>GFFSFIGEAFQGAGDMWRAYTDMKEAGWKDGDKYFHARGNYDAAQRGPGGVWAAEKISDARESFQEFFGRGHEDTMADQEANRHGRSGKDPNYYRPPGLPAKY[24x]

SAA1.1 is an acute phase protein that becomes strongly upregulated during inflammation. Chronic inflammatory conditions, such as tuberculosis, leprosy and rheumatoid arthritis, are risk factors for the development of systemic AA amyloidosis. We report three cryo-EM structures of SAA1.1-derived amyloid fibrils: one that was extracted from the diseased murine tissue and two that were formed from murine SAA1.1 protein in vitro. In vitro and ex vivo fibrils possess parallel cross-β sheets but differ in their overall topologies and fibril protein folds.

Cryo-EM reconstructions achieved spatial resolutions of 2.73 Å for morphology i and 2.95 Å for morphology ii. Morphology ii is also polar but presents C2 symmetry. It consists of two PFs that both exhibit the structure of the morphology i PF. Both fibril morphologies contain an identical protein fold. In contrast to morphology i, however, morphology ii PFs contains two non-equal protein stacks, termed here stacks a and b. They differ in their relative position in the fibril structure and at the interface between the two PFs. Lys24 (stack a) in one PF is packed against Glu25 (stack a) in the other PF. Glu8 (stack b) in one PF is opposite to Lys29 (stack a) in the other PF. In conclusion, both in vitro formed fibril morphologies contain the same fibril protein fold and differ in the PF number.Jingmenviruses are a category of emerging segmented viruses that have garnered global attention in recent years, and are close relatives of the flaviviruses in the Flaviviridae family. One of their genome segments encodes NSP1 homologous to flavivirus NS5. NSP1 comprises both the methyltransferase (MTase) and RNA-dependent RNA polymerase (RdRP) modules playing essential roles in viral genome replication and capping. The NSP1 RdRP exhibits a characteristic architectural feature commonly found in viral RdRPs, known as encircled right-hand architecture.

To gain insights into the structural characteristics of jingmenvirus NSP1, we conducted a crystallization screening experiment for three variants: FL (residues 1–915) JMTV NSP1, as well as two N-terminal truncation constructs, namely D55 (residues 56–915) and D307 (residues 308–915). Although the FL construct did not yield any crystals, the D55 and D307 constructs produced crystals with flake-like and stick-like shapes, respectively. Subsequently, the structures of native D55 and D307 were resolved through molecular replacement, utilizing the Se-Met-derived D55 structure as the search model. Due to the significant similarity between the native structures of D55 and D307, with a root-mean-square deviation (RMSD) value of merely 0.2 Å for all superimposable α-carbon atoms (with D307 structure as the reference, covering 99.5% of residues), we primarily utilize the 1.84-Å D307 structure for subsequent illustrations. The D307 structure exhibits unresolved regions, namely residues 359–361 and 388–389 in the index finger, residues 504–518 at the tip of the ring finger, residues 779–785 in the thumb loop located between α-helices 21 and 22, residues 830–836 in part of PE, and residues 912–915 at the very C-terminus. The active site is situated within the interstitial region of the three domains, encompassed by seven RdRP catalytic motifs A-G. Even if compared with the most resembling flavivirus RdRP structure obtained using an MTase-less DENV2 NS5 (39), the right-hand structure of JMTV NSP1 RdRP exhibits a tighter grip with the top of both thumb and fingers domains (primarily pinky finger) moving inward for 4–5 Å. The NSP1 RdRP closely resembles the RdRPs found in the Flavivirus genus, which includes the N-terminal extension (NE) and one-segment PE, both of which are characteristic features of flaviviruses. The JMTV PE exhibits partial disorder, but it is characterized by a one-segment structure that closely resembles the PEs of flaviviruses in terms of length and structure. However, it is worth noting that the linker region in JMTV NE is approximately 10 residues longer compared to that of flaviviruses, and it forms a cofold with the palm domain. Remarkably, the quantity of intermediate products (specifically, 4-mer in the P2-to-P5 assay and 4-mer/5-mer in the P2-to-P7 assay) generated by NSP1 D307 was observed to be greater than that of FL NSP1 (when comparing lanes 13–21/22–30 and lanes 53–61/62–70).

> MEWTAEAVIEGCAPLTPLNMTRSIAEMHMEYPPLGITRFFKELGYKIAKKKGSEGTRKNRFVGQLIEPLRRVLERHHLFGAWQLTSTTPRAVFNMFRSKVDRAPVELHSHYPGLKKMYDILADLWLERYGSMKRLTEEEMASAINRRGAMGYQMDNRNYGDLGAYWDSGDWRQDVNTFKRALLSGTPTHAVYNTTAKKEKTKNLTRQVNKGSRIIQYLPADARLYELKVLGGLHKYLEKCGWSVAGQGLYKYGDRVKKSMDATGAAISEDVAGWDTKISKGLLTLESHMFTKLAEDEEMAREIHHLYRLYADPHMVVQREIEGEVHDVLLRGRGQVSSGRQPTYAANTITNFITTTYGMAVTLGIPEADWPRLIRDLTDERGNRRLLVSGDDKVLFLRGDEARVYASSAYRISNDMGLVRKDMALEQESEIIVDVKEISFCSHRYWPVKYGNEIHYMPVRDVGEIFAKATMALGVYKDDMTQEAWARVQGLNMLVNYHHIPECRMLALAILSVTRIGLNLKGITKGWMMSTEWLRDDLAPDTIHALITEGRTSGWDQLGYVDFKDRKGILLRPDTNYKNWRRDLPEKVRQLREDGQYKDWLQKMAVFGGSSSGTHHHHHH>[3x]GMSQPKKRKLESGGGGEGGEGTEEEDGAEREAALERPRRTKRERDQLYYECYSDVSVHEEMIADRVRTDAYRLGILRNWAALRGKTVLDVGAGTGILSIFCAQAGARRVYAVEASAIWQQAREVVRFNGLEDRVHVLPGPVETVELPEQVDAIVSEWMGYGLLHESMLSSVLHARTKWLKEGGLLLPASAELFIVPISDQMLEWRLG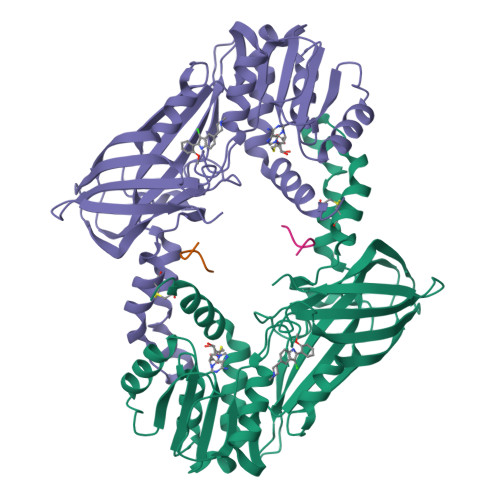FWSQVKQHYGVDMSCLEGFATRCLMGHSEIVVQGLSGEDVLARPQRFAQLELSRAGLEQELEAGVGGRFRCSCYGSAPMHGFAIWFQVTFPGGESEKPLVLSTSPFHPATHWKQALLYLNEPVQVEQDTDVSGEITLLPSRDNPRRLRVLLRYKVGDQEEKTKDFAMED> SALQDLLRTL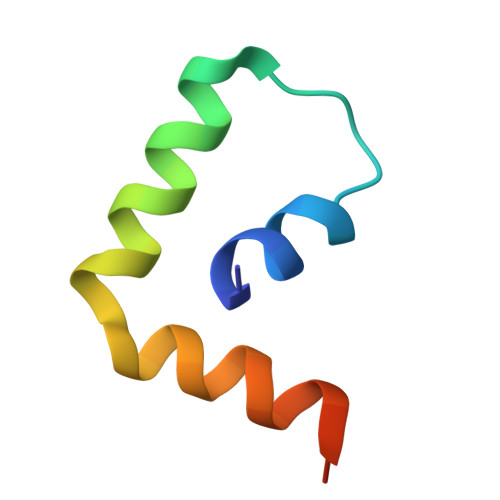KSPSSPQQQQQVLNILKSNPQLMAAFIKQRTAKYVAN3-[(2~{S},3~{R},4~{R})-4-azanyl-2-carboxy-pyrrolidin-3-yl]propyl-$l^{3}-oxidanyl-bis(oxidanyl)boron | C8 H18 B N2 O5 | 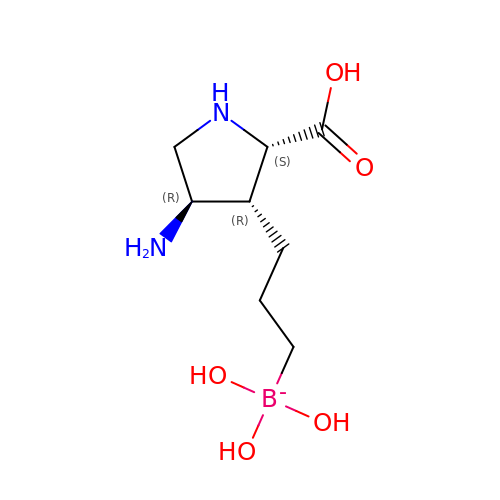LCXKCSYMGHLIAH-VQVTYTSYSA-N>MRRVVVTGLGALTPIGVGQEAFHKAQLAGKSGVRPITRFDASALPVRIAAEVDVDPGAYLDRKELRRLDRFVQYALIAAQLALEDAGLKPEDLDPERVGTLVGTGIGGMETWEAQSRVFLERGPNRISPFFIPMMIANMASAHIAMRYGFTGPSSTVVTACATGADALGSALRMIQLGEADLVLAGGTEAAITPMAIGAFAVMRALSTRNEEPEKASRPFTLSRDGFVMGEGAGVLVLEAYEHAKKRGARIYAELVGFGRSADAHHITEPHPEGKGAALAMARALKDAGIAPEQVGYINAHGTSTPVGDRAEVLAIKRVFGDHAKRLMVSSTKSMIGHLLGAAGAVEAIATVQALYHGVIPPTINLEDPDPELDLDFVPEP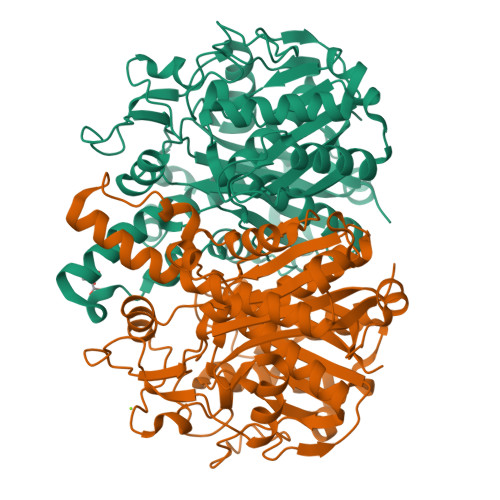REAKVDYALSNSFAFGGHNAVLAFKRV[2x]>MKFKHQGLVADLLPNIRVMQGVGHFMFNYYSEGKKFPHRIYCIVTLLLLLLQYGMMAVNLMMESDDVDDLTANTITMLFFLHPIVKMIYFPVRSKIFYKTLAIWNNPNSHPLFAESNARFHALAITKMRRLLFCVAGATIFSVISWTGITFIEDSVKRITDPETNETTIIPIPRLMIRTFYPFNAMSGAGHVFALIYQFYYLVISMAVSNSLDVLFCSWLLFACEQLQHLKAIMKPLMELSATLDTVVPNSGELFKAGSADHLRESQGVQPSGNGDNVLDVDLRGIYSNRQDFTATFRPTAGTTFNGGVGPNGLTKKQEMLVRSAIKYWVERHKHVVRLVTAVGDAYGVALLLHMLTTTITLTLLAYQATKVNGVNVYAATVIGYLLYTLGQVFLFCIFGNRLIEESSSVMEAAYSCHWYDGSEEAKTFVQIVCQQCQKAMSISGAKFFTVSLDLFASVLGAVVTYFMVLVQLK[3x];> MARLVLHEVRYVLMAMLYISRGMAKQIQNSTIDLYVYWFLTFIPIASLCVPQFTYLVVDTKSLIDFISVLVPITEILLTNGKMIICNVKRGKIINLINQVQVAWDECAKSEHLEIQTLITATAKKTKIFVIIYTTSFLLICVEYSSMPLFKLIYHSAVYGKQSNYTIALPYLSRFAYSTESTTSFAWTYFFILLGVYLLALTLSGFDSLFATLVMHVKMMFKVLKFEIEQLGLDLSAGKSHVELQAKLKQIILKHKTNLSLIEQLEDGFSFFLMAQFLTSS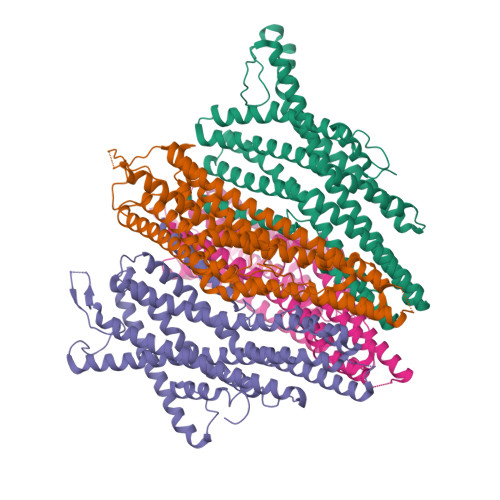ILVCVVLYELTMVFGWNEDTFKTVTYLPGAILQLFLFCWYAQQITEEARLVSDHIYNIPWYLADPKLQKDILTFMVKAQKPTGVTASKFYMVTLQTFQRISSTSYSYFTLLQTINQQ>[10x]MSLSVKILFKNATVFPITSRPFKGDVLVSNGKVEKVGENIEDPDAEIVDLTGKFLFPGFVDAHSHIGLFEEGVGYYYSDGNEATDPVTPHVKALDGFNPQDPAIERALAGGVTSVMIVPGSANPVGGQGSVIKFRSIIVEECIVKDPAGLKMAFGENPKRVYGERKQTPSTRMGTAGVIRDYFTKVKNYMKKKELAQKEGKEFTETDLK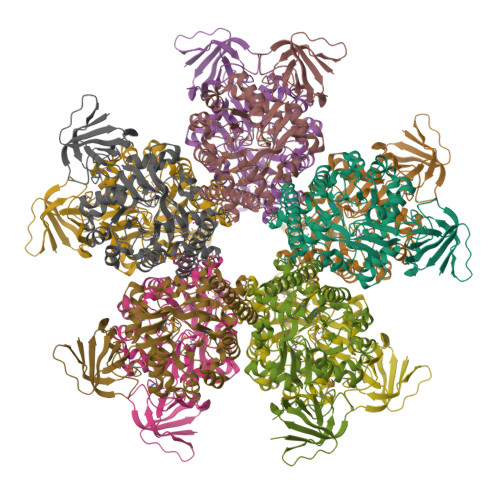MEVGEMVLRKKIPARMHAHRADDILTAIRIAEEFGFNLVIEHGTEAYKISKVLAEKKIPVVVGPLLTFRTKLELKDLTMETIAKLLKDGVLIALMCDHPVIPLEFATVQAATAMRYGAKEEDLLKILTVNPAKILGLEDRIGSIEPGKDADLVVWSGHPFDMKSVVERVYIDGVEVFRREGHHHHHH> MGHHHHHHMKQKIVSMEEAISHVKDGMTVHIGGFIACGTPESIITALIEKGVKDLTIVANDTGLIDKGIGRLVVN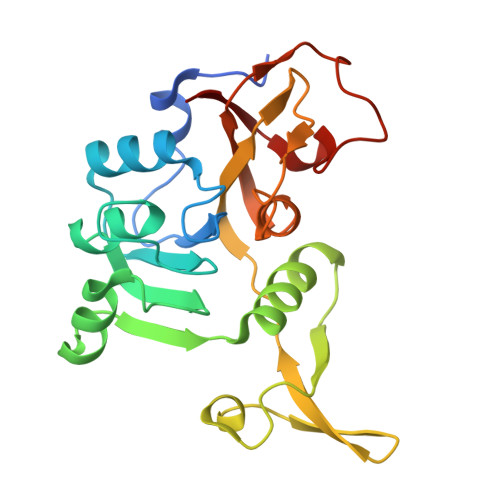NQVKKVIASHIGTNPETGRRMQSGEMEVELVPQGTLAERVRAAGYGLGGILTPTGLGTIVQEGKQIINVDGKDYLLEKPIKADVALIFGTKVDELGNVICEKTTKNFNPLMATAADVVIVEALEIVPAGSLSPEHLDISRIFIDYIVKSK> DYTNYTNKEMQAVTIAKQIKNGQVVTVGTGLPLIGASVAKRVYAPDCHIIVESGLMDCSPVEVPRSVGDLRFMAHCGCIWPNVRFVGFEINEYLHKANRLIAFIGGAQIDPYGNVNSTSIGDYHHPKTRFTGSGGANGIATYSNTIIMMQHEKRRFMNKIDYVTSPGWIDGPGGRERLGLPG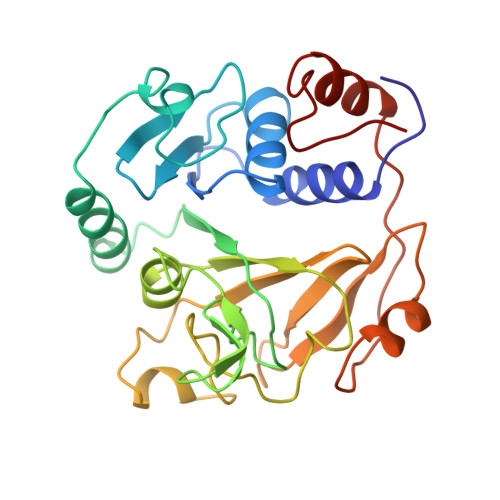DVGPQLVVTDKGILKFDEKTKRMYLAAYYPTSSPEDVLENTGFDLDVSKAVELEAPDPAVIKLIREEIDPGQAFIQVP>[4x]MKRAVITGLGIVSSIGNNQQEVLASLREGRSGITFSQELKDSGMRSHVWGNVKLDTTGLIDRKVVRFMSDASIYAFLSMEQAIADAGLSPEAYQNNPRVGLIAGSGGGSPRFQVFGADAMRGPRGLKAVGPYVVTKAMASGVSACLATPFKIHGVNYSISSACATSAHCIGNAVEQIQLGKQDIVFAGGGEELCWEMACEFDA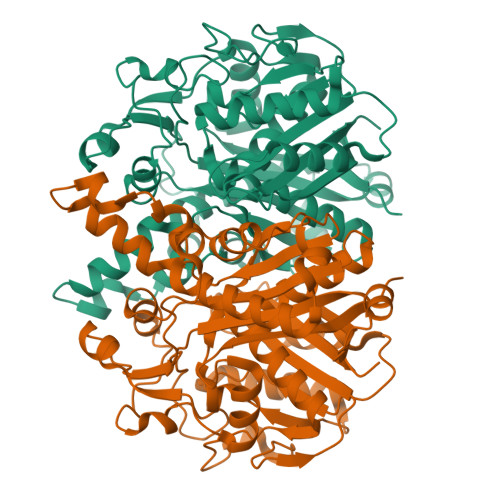MGALSTKYNDTPEKASRTYDAHRDGFVIAGGGGMVVVEELEHALARGAHIYAEIVGYGATSDGADMVAPSGEGAVRCMKMAMHGVDTPIDYLNSHGTSTPVGDVKELAAIREVFGDKSPAISATKAMTGHSLGAAGVQEAIYSLLMLEHGFIAPSINIEELDEQAAGLNIVTETTDRELTTVMSNSFGFGGTNATLVMRKLKD One widely occurring ribonuclease with such multi-functional versatility is polynucleotide phosphorylase, a phosphorolytic exoribonuclease (PNPase; polyribonucleotide nucleotidyltransferase; EC 2.7.7.8).5,6 PNPase processively cleaves single-stranded RNA substrates in the 3′-to-5′ direction using inorganic phosphate to attack the phosphoester linkage at the 3′ terminus and liberate nucleoside diphosphate. E. coli PNPase core forms a homotrimer with a ring-like architecture that encloses a large central channel. The two RNase PH-like domains within each protomer are spatially related by a pseudo-dyad axis, so that the PNPase trimer has approximate dihedral symmetry D3. In the current study, we solved several crystal structures of E. coli PNPase core bound to its cognate RNase E micro-domain, including a complex with O2′-methyl-modified RNA bound and another with manganese in the active site.

The RNase E micro-domain is also well resolved in the rhombohedral crystal form with Mn2+ but was poorly resolved in the second rhombohedral form grown in the absence of the metal. In the RNA-free form, however, the helical domain is partially disordered, which suggests that it is highly dynamic and may potentially become more structurally defined upon substrate binding. In comparing the RNA-free structures of the PNPase core, we observe that the FFRR loop is dynamic, as we find that it constricts the pore in one apo form, but it is disordered in a second crystal form. We observe also that RNA binding at the aperture requires two channel-loops and may pre-organise one of those to engage another RNA base as the oligonucleotide is translocated along the pore. It is likely that the S1 and KH domains may also affect the conformational adjustments, since a comparison of the structures of full-length E. coli PNPase and PNPase core in the RNA-free forms shows that the central aperture is expanded in the latter.

> MLNPIVRKFQYGQHTVTLETGMMARQATAAVMVSMDDTAVFVTVVGQKKAKPGQDFFPLTVNYQERTYAAGRIPGSFFRREGRPSEGETLIARLIDRPIRPLFPEGFVNEVQVIATVVSVNPQVNPDIVAMIGASAALSLSGIPFNGPIGAARVGYINDQYVLNPTQDELKESKLDLVVAGTEAAVLMVESEAELLSEDQMLGAVVFGHEQQQVVIQNINELVKEAGKPRWDWQPEPVNEALNARVAALAEARLSDAYRITDKQERYAQVDVIKSETIATLLAEDETLDENELGEILHAIEKNVVRSRVLAGEPRIDGREKDMIRGLDVRTGVLPRTHGSALFTRGETQALVTATLGTARDAQVLDELMGERTDTFLFHYNFPPYSVGETGMVGSPKRREIGHGRLAKRGVLAVMPDMDKFPYTVRVVSEITESNGSSSMASVCGASLALMDAGVPIKAAVAGIAMGLVKEGDNYVVLSDILGDEDHLGDMDFKVAGSRDGISALQMDIKIEGITKEIMQVALNQAKGARLHILGVMEQAINAPRGDIS> MSAE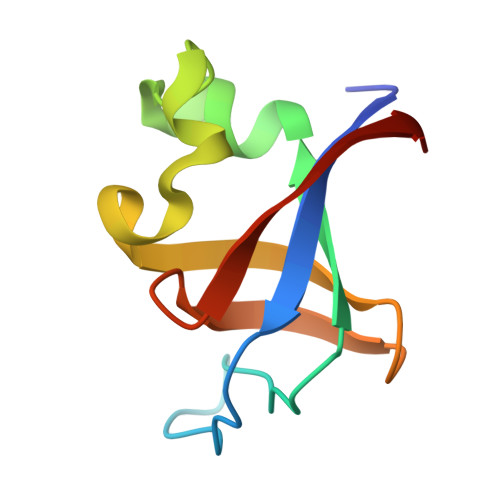GYQYRALYDYKKEREEDIDLHLGDILTVNKGSLVALGFSDGQEARPEEIGWLNGYNETTGERGDFPGTYVEYIGRKKIS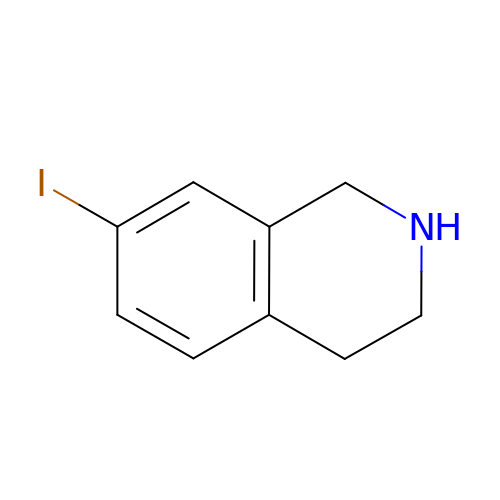7-IODO-1,2,3,4-TETRAHYDRO-ISOQUINOLINE | C9 H10 I N | FFCFXJXBXUOFIU-UHFFFAOYSA-N> KPFSLPILTISELTNSRFPAPIDSLFTAQNNNLNVQCQNGRCTLDGELQGTTQLLPSGICAFRGRLTADVDGSHDDRWHMQLTNLNGTPFDPTEDVPAPLGTPDFTGLLFGVASQRNVGSNPNTTRAHEAVISTTSSQFVPKLGSVNFGSTSTDFQLQQPTKFTPVGIKIESGHEFDQWALPRYSGHLTLNMNLAPPIAPNFPGEQLLFFRSNVPCAGGVSDGVIDCLLPQEWIQHFYQESAPSQSDVALIRYVNPDTGRTLFEAKLHRTGYITVAHSGDYPLVVPSNGYFRFDSWVNQ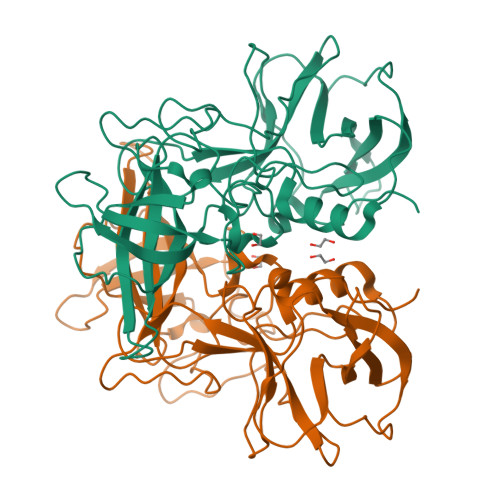FYSLAPM> MKIVSWNINGIRATRVGLKETLDSLDADIICLQETKVTRDLLDEPSAIVEGYNSYFSFSRVRSGYSGVATFCKSSTTPQAAEEGLSGVFCNRTGSVGCYGNTEQFLEEELQSLDQEGRAVLTQHRILNCEDKEETLTVINVYCPRADPEKPERKTYKLRFYHLLQTRAEAILQNGGHVIILGDVNTSHRPLDHCDPTDLETFEENPGRQWLNQFLGDPIPSQKGDSETVMPPSAGSGLFYDSFR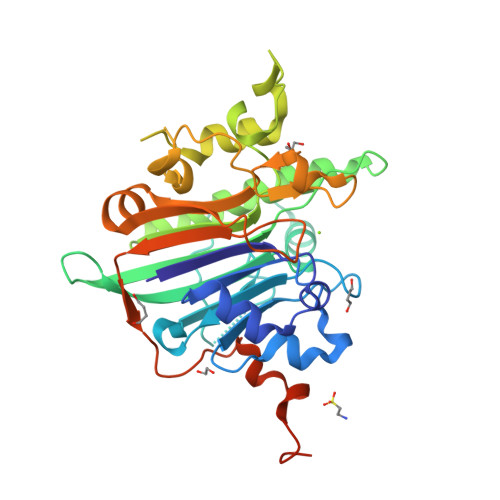YFHPTQKNAFTCWCSASGARQTNYGTRIDYILGNRELVESEFLDSVIMPEVEGSDHCPVKAFMKCQPIAANKCPPLCTKYLPEFAGRQQKLLQFLVKKENTLGNTTEESSE>MSKPQPIAAANWKCNGSQQSLSELIDLFNSTSINHDVQCVVASTFVHLAMTKERLSHPKFVIAAQNAIAKSGAFTGEVSLPILKDFGVNWIVLGHSERRAYYGETNEIVADKVAAAVASGFMVIACIGETLQERESGRTAVVVLTQIAAIAKKLKKADWAKVVIAYEPVWAI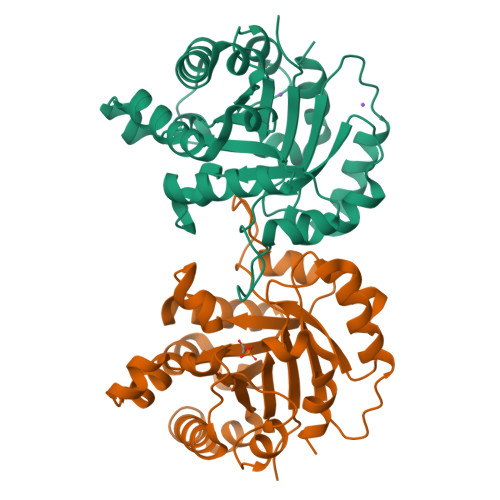GTGKVATPQQAQEAHALIRSWVSSKIGADVAGELRILYGGSVNGKNARTLYQQRDVNGFAVGGASLKPEFVDIIKATQ[4x]> MAPVKVFGPAMSTNVARVTLCLEEVGAEYEVVNIDFNTMEHKSPEHLARNPFGQIPA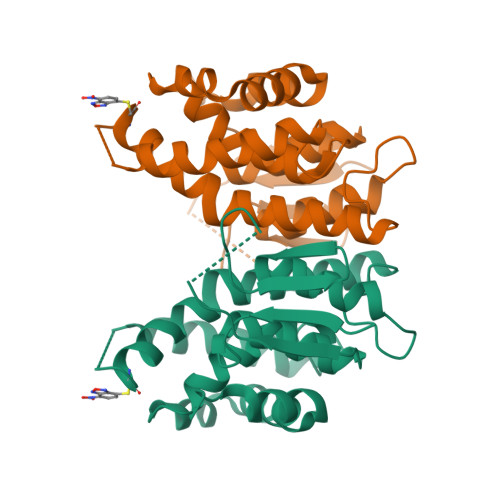FQDGDLLLWESRAISKYVLRKYKTDEVDLLRESNLEEAAMVDVWTEVDAHTYNPALSPIVYQCLFNPMMRGLPTDEKVVAESLEKLKKVLEVYEARLSKHSYLAGDFVSFADLNHFPYTFYFMATPHAALFDSYPHVKAWWDRLMARPAVKKIAATMVPPKACLFAESLEKLKKVLEVYEARLSKHSYLAGDFVSFADLNHFPYTFYFMATPHAALFDSYPHVKAWWDRLMARPAVKKIAATMVPPKA> MASIHSLLSACQTTPRDVAEPAQVRIALWDKWLAPVTPDNPAGDDAGYDDDFQQMREEVNKLSGADAGIVSQLAEKLLTTRTKDIRVATWYIWARLRQDGEKGLADGLELLTGLLQRFGEHLHPQRSRARKAALEWLCSARILDSLSLYPEVVKADTLRIAGALWLAEQTFTDEASAPVLNGLYQALENRLMKAGGVDAVVPQEAAAPAPTVTSGSVMALSAITSGQELLSQARVLAKYLRDQPEGWLAAHRLMKSVRHDTLHQLPPLSADGRTRIAPPGPDRRASLKRLYLQQNWLSLLEQCDDMFARGASHLWLD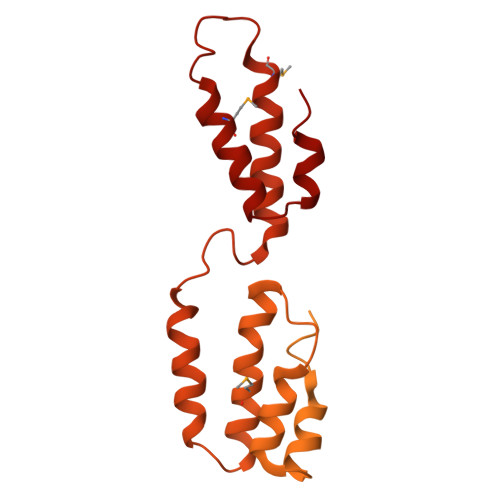LQWYIHQALLQTGKENYAAIIQYDLKGLLLRLPGLETLAFNDGMPFADDVTLSWIQQQVMECGERWAEEPSVTITAAPGDNDILSLEPEALQIADNEGTEAALSWLQARPGIQSDRSNWLLRLLMARVAEQTGKNDLALHLLAELDERATRLTLSQWEPELVFEVKARRLKLLRMKSAKTESDRVRLQPDMEHLLAGLIAIDAARAAVLCNSGSS2-chloro-N-methyl-N-[3-(10H-phenothiazin-10-yl)propyl]acetamide 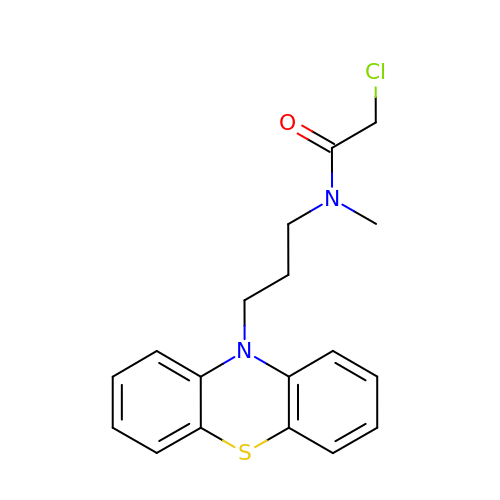| C18 H19 Cl N2 O S | DGIQIBHRQRNGPY-UHFFFAOYSA-N> MPISAGSLKTRLLAQRRTSGTDDWGAPVQGWSDLGLFSGDVKNDTGLGAIRTAAGSGLPASIAKYSIKVRSEVIRRWSINSADRIIGRLPFSTQEMVFSVTGVISDFAD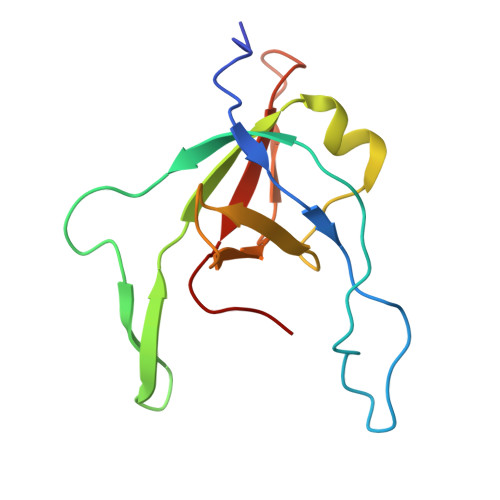PSMAYILVEAGADEQ>MAKKTGAKYPKSLLSLPLVGSLPFLPRHGHMHNNFFKLQKKYGPIYSVRMGTKTTVIVGHHQLAKEVLIKKGKDFSGRPQMATLDIASNNRKGIAFADSGAHWQLHRRLAMATFALFKDGDQKLEKIICQEISTLCDMLATHNGQSIDISFPVFVAVTNVISLICFNTSYKNGDPELNVIQNYNEGIIDNLSKDSLVDLVPWLKIFPNKTLEKLKSHVKIRNDLLNKILENYKEKFRSDSITNMLDTLMQAKMNSDNGNAGPDQDSELLSDNHILTTIGDIFGAGVETTTSVVKWTLAFLLHNPQVKKKLYEEIDQNVGFSRTPTISDRNRLLLLEATIREVLRLRPVAPMLIPHKANVDSSIGEFAVDKGTEVIINLWALHHNEKEWHQPDQFMPERFLNPAGTQLISPSVSYLPFGAGPRSCIGEILARQELFLIMAWLLQRFDLEVPDDGQLPSLEGIPKVVFLIDSFKVKIKVRQAWREAQAEGSTHHHH[4x]

Alkyl isonitriles, R—NC, have previously been shown to ligate the heme (haem) iron of cytochromes P450 in both accessible oxidation states (ferrous, Fe2+, and ferric, Fe3+). Herein, the preparation of four steroid-derived isonitriles and their interactions with several P450s, including the steroidogenic CYP17A1 and CYP106A2, as well as the more promiscuous drug metabolizers CYP3A4 and CYP2D6, is described. It was found that successful ligation of the heme iron by the isonitrile functionality for a given P450 depends on both the position and stereochemistry of the isonitrile on the steroid skeleton. A crystallographic structure of CYP17A1 with an isonitrile derived from pregnanalone further confirmed the interaction and identified the absolute stereochemistry of the bound species.

Co-crystallization of CYP17A1 with the tighter-binding epimer of 1 and subsequent X-ray diffraction analysis revealed that this is the 20-(R) epimer and confirmed formation of a bond between the carbon atom of the isonitrile functionality and the heme Fe. The positioning of 1 in the active site is well-defined by the electron density, rising ~60° to the heme normal, orienting the C20 isonitrile group directly above the Fe. The C3 formyl ester substituent projects between N202, R239, and several waters, components that typically interact with both steroidal and nonsteroidal CYP17A1 ligands. The position of the heme-ligating isonitrile of 1 is similar to that of the pyridine nitrogen of abiraterone in those structures. As is typical for CYP17A1 structures, two of the four monomers in the asymmetric unit have a slightly different conformation of the F/G and N-terminal regions. Indeed, a second copy of 1 is bound in this peripheral site. Binding of this second copy of the ligand is also consistent with the steep slope observed in the inhibition experiment, suggesting a 2:1 stoichiometry, while the spectral shift binding assay only reports on the ligand molecule binding in the active site where it can cause a spin shift. However, in neither conformation does the binding of 20-(R)-1 result in significant changes to the overall protein fold compared to structures with steroidal substrates or other steroidal inhibitors. The structure suggests a possible reason why compounds 2 and 3 with isonitrile functionality at C17 do not ligate the heme iron, while 1 with a C20 isonitrile does (vide supra).1-[2-(2-Hydroxy-ethyl)-phenyl]-3-(3-trifluoromethoxy-phenyl)-urea 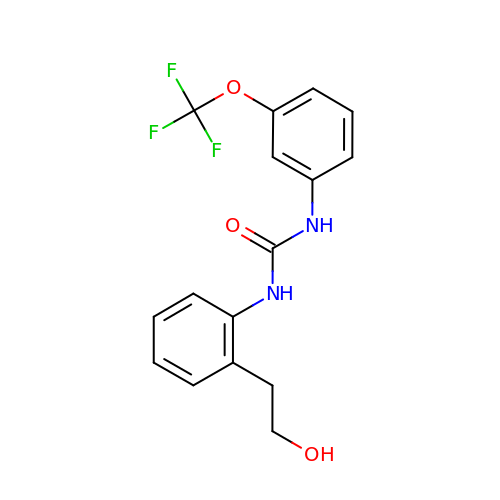| C16 H15 F3 N2 O3 | QYTRNJRTLNCHSJ-UHFFFAOYSA-N>[2x]MWQQAIGDALGITARNLKKFGDRFPHVSDGSNKYVLNDNTDWTDGFWSGILWLCYEYTGDEQYREGAVRTVASFRERLDRFENLDHHDIGFLYSLSA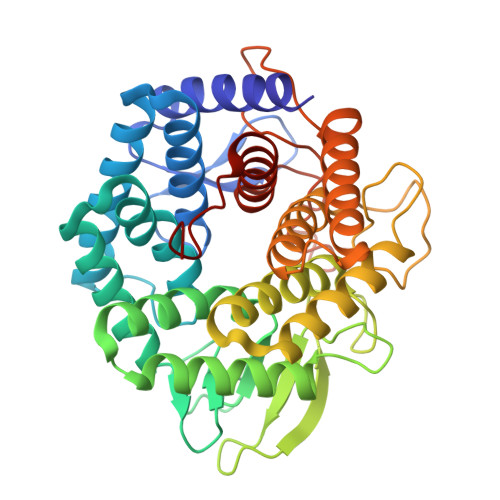KAQWIVEKDESARKLALDAADVLMRRWRADAGIIQAWGPKGDPENGGRIIIDCLLNLPLLLWAGEQTGDPEYRRVAEAHALKSRRFLVRGDDSSYHTFYFDPENGNAIRGGTHQGNTDGSTWTRGQAWGIYGFALNSRYLGNADLLETAKRMARHFLARVPEDGVVYWDFEVPQEPSSYRDSSASAITACGLLEIASQLDESDPERQRFIDAAKTTVTALRDGYAERDDGEAEGFIRRGSYHVRGGISPDDYTIWGDYYYLEALLRLERGVTGYWYERGR> EYRIDRVRLFVDKLDNIAQVPRV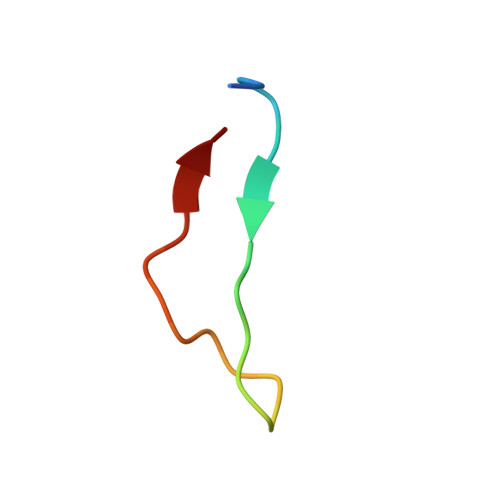G>MSSLLNSLLPEYFKPKTNLNINSSRVQYGFNARIDMQYEDDSGTRKGSRPNAFMSNTVAFIGNYEGIIVDDIPILDGLRADIFDTHGDLDMGLVEDALSKSTMIRRNVPTYTAYASELLYKRNLTSLFYNMLRLYYIKKWGSIKYEKDAIFYDNGHACLLNRQLFPKSRDASLESSLSLPEAEIAMLDPGLEFPEEDVPAILWHGRVSSRATCILGQACSEFAPLAPFSIAHYSPQLTRKLFVNAPAGIEPSSGRYTHEDVKDAITILVSANQAYTDFEAAYLMLAQTLVSPVPRTAEASAWFINAGMVNMPTLSCANGYYPALTNVNPYHRLDTWKDTLNHWVAYPDMLFYHSVAMIESCYVELGNVARVSDSDAINKYTFTELSVQGRPVMNRGIIVDLTLVAMRTGREISLPYPVSCGLTRTDALLQGTEIHVPVVVKDIDMPQYYNAIDKDVIEGQETVIKVKQLPPAMYPIYTYGINTTEFYSDHFEDQVQVEMAPIDNGKAVFNDARKFSKFMSIMRMMGNDVTATDLVTGRKVSNWADNSSGRFLYTDVKYEGQTAFLVDMDTVKARDHCWVSIVDPNGTMNLSYKMTNFRAAMFSRNKPLYMTGGSVRTIATGNYRDAAERLRAMDETLRLKPFKITEKLDFRVAAYAIPSLSGSNMPSLHHQEQLQISEVDAEPINPIGEDELPPDIE[110x]

L-BC virus persists in the budding yeast Saccharomyces cerevisiae, whereas other viruses from the family Totiviridae infect a diverse group of organisms including protists, fungi, arthropods, and vertebrates. Totiviridae is a family of viruses with monopartite double-stranded RNA (dsRNA) genomes, which contain two open reading frames encoding the capsid protein and the RNA-dependent RNA-polymerase (RdRp). The capsid of L-BC is organized with icosahedral symmetry with two subunits of capsid protein, named A and B, forming the icosahedral asymmetric unit. Decamers of capsid proteins are stabilized by domain swapping of the C-termini of subunits located around icosahedral fivefold axes.

The two-dimensional classification of L-BC particle images identified a subpopulation of 9% of particles missing segments of their capsids. Asymmetric reconstruction of the open particles lacking a large segment of its capsid with the opening centered around a fivefold axis. The borders of the capsid opening are formed by poorly resolved density which may be caused by the limited number of images (1120) available for the reconstruction or by variations in the structure of individual open particles. The structures of capsid proteins from the empty particle were fitted into the other reconstructions. The existence of the open particles together with domain swapping within a decamer provides evidence that Totiviridae capsids assemble from the decamers of capsid proteins. Furthermore, the open particles may be assembly intermediates that are prepared for the incorporation of the virus (+) strand RNA.> GGLEKDFLPLYFGWFLTKKSSETLRKAGQVFLEELGNHKAFKKELRHFISGDEPKEKLELVSYFGKRPPGVLQCTTKFCDYGKAAGAEEYAQQEVVKRSYGKAFKLSISALFVTPKTAGAQVVLTDQELQLWPSDLDKPSASEGLPPGSRAQVTLGCAADVQPVQTGLDLLDILQQVKGGSQGEAVGELPRGKLYSLGKGRWMLSLTKKMEVKAIFTGYYG

2′,3′-cyclic nucleotide 3′-phosphodiesterase (CNPase) comprises 4% of total myelin protein in the central nervous system (CNS), being the most abundant CNS non-compact myelin protein4. CNPase consists of an N-terminal polynucleotide kinase-like domain10, a catalytic phosphodiesterase domain11, and a membrane-anchored C-terminal tail, which contains a cysteine residue that undergoes isoprenylation. The catalytic domain enables the rapid hydrolysis of nucleoside 2′,3′-cyclic phosphates to nucleoside 2′-phosphates. The CNPase catalytic site, lying in a groove between two lobes, has pseudo two-fold symmetry and contains two apposing His-X-Thr-X (X denotes a hydrophobic residue) motifs, characteristic for 2H phosphoesterases 113537.

In mouse CNPase, this is done by His230, Thr232, His309, and Thr311, in a manner, where a nucleophilic water molecule activated by His309 can attack the cyclic phosphate and a pentavalent transition state is formed. Mutation of active-site histidine residues (H230Q, H230S, H309Q, H309S, and H230Q/H309Q double mutant) abolishes CNPase activity. Overall, the structures of H230S, H309S, H230Q, H309Q, and H230Q/H309Q are highly similar. However, only H230S and H309S could be used to trap nucleotide ligands within the active site, whereas H309Q and the H230Q/H309Q double mutant could not. The results indicate that all the variants were correctly folded and heat-stable, with the largest destabilization, 8–9 °C, caused by the H230Q/H309Q double mutation. The catalytic motif, thus, is also important for CNPase stability.3-(3-fluorophenyl)-1H-pyrazole | C9 H7 F N2 | 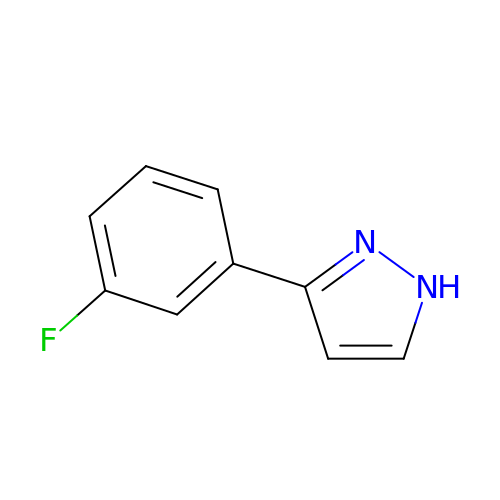WKIRCCSDGDQJJF-UHFFFAOYSA-N>MGHHHHHHHHHHSSGHENLYFQGHMANRNVEKLASIDAQLRLLVPGKVSEDDKLVEYDALLLDKFLDILQDLHGEDLKEAVQQCYELSAEYEGKHDPKKLEELGSLLTSLDTGDSIVIAKAFSHMLNLANLAEELQIAYRRRIKLKSGDFADEANATTESDIEETFKRLVHKLNKSPEEVFDALKNQTVELVLTAHPTQSVRRSLLQKHGRIRNCLAQLYAKDITPDDKQELDEALHREIQAAFRTDEIRRTPPTPQDEMRAGMSYFHETIWKGVPKFLRRVDTALKNIGINERFPYNAPLIQFSSWMGGDRDGNPRVTPEVTRDVCLLARMMTSNMYFSQIEDLMIEMSMWRCNSELRVRAEELYRTARKDVKHYIEFWKRIPPNQPYRVILGDVRDKLYNTRERSRHLLVDGKSDIPDEAVYTNVEQLLEPLELCYRSLCDCGDHVIADGSLLDFLRQVSTFGLSLVKLDIRQESDRHTEVLDAITQHLGIGSYREWSEEKRQEWLLAELSGKRPLIGPDLPKTEEVKDCLDTFKVLAELPSDCFGAYIISMATSTSDVLAVELLQREYHIKHPLRVVPLFEKLADLEAAPAAMTRLFSMDWYRNRIDGKQEVMIGYSDSGKDAGRFSAAWQLYKTQEQIVKIAKEFGVKLVIFHGRGGTVGRGGGPTHLALLSQPPDTINGSLRVTVQGEVIEQSFGEEHLCFRTLQRFCAATLEHGMNPPISPRPEWRELMDQMAVVATEEYRSVVFKEPRFVEYFRLATPELEFGRMNIGSRPSKRKPSGGIESLRAIPWIFSWTQTRFHLPVWLGFGAAFKHAIQKDSKNLQMLQEMYKTWPFFRVTIDLVEMVFAKGN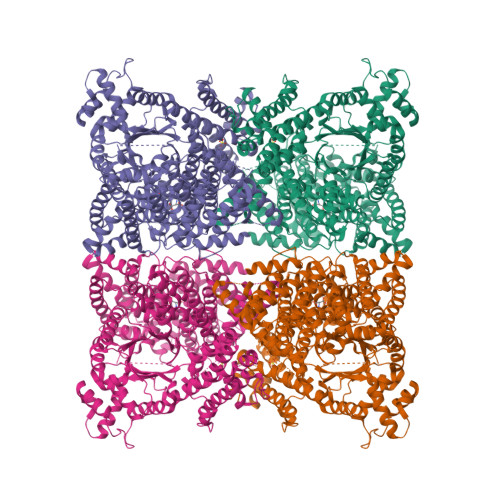PGIAALNDKLLVSEDLRPFGESLRANYEETKNYLLKIAGHKDLLEGDPYLKQGIRLRDPYITTLNVCQAYTLKRIRDPNYHVTLRPHISKEYAAEPSKPADELIHLNPTSEYAPGLEDTLILTMKGIAAGMQNTG[2x]>MLPGTFFEVLKNEGVVAIATQGEDGPHLVNVWNSYLKVLDGNRIVVPVGGMHKTEANVARDERVLMTLGSRKVAGRNGPGTGFLIRGSAAFRTDGPEFE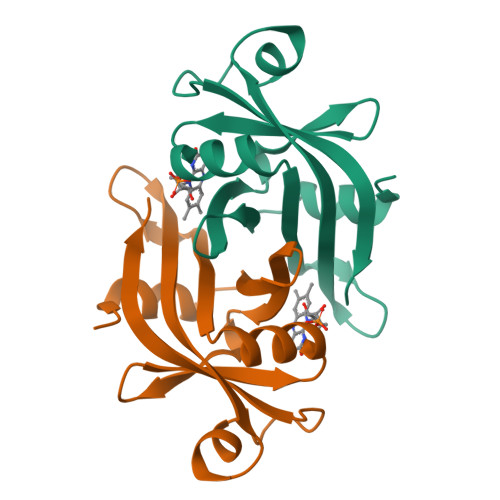AIARFKWARAALVITVVSAEQTL[2x]>[4x]MKATEQHYSIKEAMLFSQRIAQLSKALWKSIEKDWQRWIK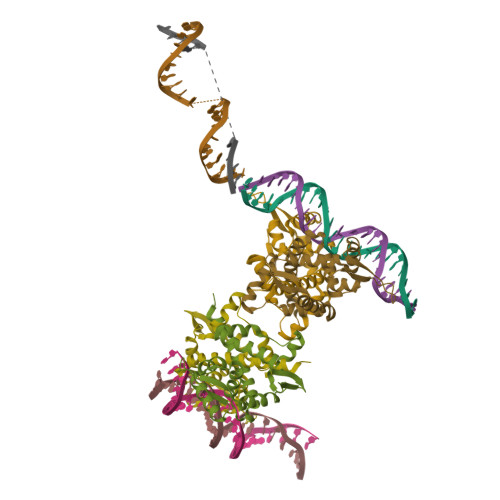PFDLNINEHHILWIAYHFKGASISEIAKFGVMHVSTAFNFSKKLEEKGLLSFSKKQDDKRNTYIELTEKGEEVLMKLMETYDPTKNAVFNGALPLRELYGKFPEILEMMCIVRNIYGDDFMEIFERAFENIKEDFIEQDGKLVKRKPKTEEHEKELASQANHHHHHH>[2x]DDATADSRKTYTLTDYLKNTYRLKLYSLRWIS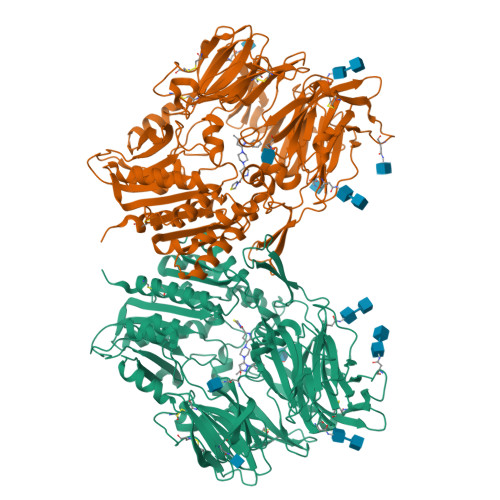DHEYLYKQENNILVFNAEYGNSSVFLENSTFDEFGHSINDYSISPDGQFILLEYNYVKQWRHSYTASYDIYDLNKRQLITEERIPNNTQWVTWSPVGHKLAYVWNNDIYVKIEPNLPSYRITWTGKEDIIYNGITDWVYEEEVFSAYSALWWSPNGTFLAYAQFNDTEVPLIEYSFYSDESLQYPKTVRVPYPKAGAVNPTVKFFVVNTDSLSSVTNATSIQITAPASMLIGDHYLCDVTWATQERISLQWLRRIQNYSVMDICDYDESSGRWNCLVARQHIEMSTTGWVGRFRPSEPHFTLDGNSFYKIISNEEGYRHICYFQIDKKDCTFITKGTWEVIGIEALTSDYLYYISNEYKGMPGGRNLYKIQLSDYTKVTCLSCELNPERCQYYSVSFSKEAKYYQLRCSGPGLPLYTLHSSVNDKGLRVLEDNSALDKMLQNVQMPSKKLDFIILNETKFWYQMILPPHFDKSKKYPLLLDVYAGPCSQKADTVFRLNWATYLASTENIIVASFDGRGSGYQGDKIMHAINRRLGTFEVEDQIEAARQFSKMGFVDNKRIAIWGWSYGGYVTSMVLGSGSGVFKCGIAVAPVSRWEYYDSVYTERYMGLPTPEDNLDHYRNSTVMSRAENFKQVEYLLIHGTADDNVHFQQSAQISKALVDVGVDFQAMWYTDEDHGIASSTAHQHIYTHMSHFIKQCFSLPHHHHHH> SPSRVLQAEELHEKALDPFLLQAEFFEIPMNFVDPKEYDIPGLVRKNRYKTILPNPHSRVCLTSPDPDDP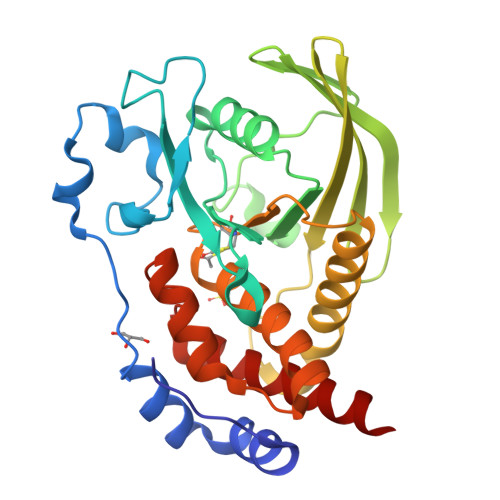LSSYINANYIRGYGGEEKVYIATQGPIVSTVADFWRMVWQEHTPIIVMITNIEEMNEKCTEYWPEEQVAYDGVEITVQKVIHTEDYRLRLISLKSGTEERGLKHYWFTSWPDQKTPDRAPPLLHLVREVEEAAQQEGPHCAPIIVHCSAGIGRTGCFIATSICCQQLRQEGVVDILKTTCQLRQDRGGMIQTCEQYQFVHHVMSLYEKQLSH A canonical two-component system consists of a homodimeric sensor histidine kinase (HK) and its cognate response regulator (RR). In the phosphotransfer reaction, the phosphate is relayed to a conserved aspartate residue within a receiver (REC) domain of the RR. By pursuing an integrated biochemical and structural strategy, we show that despite close homology, Agp1 acts as a histidine kinase whereas DrBphP functions as a light-activated phosphatase. Our results now settle this long-standing debate and show that DrBphP is a biochemically active protein that dephosphorylates the DrRR, rather than phosphorylating it.

As DrBphP and Agp1 strikingly differed in their enzymatic activity and interactions, we next asked whether these differences could be explained by the structure of the interface between the DHp and RR. To model this interface with confidence, we solved the crystal structure of the response regulator from D. radiodurans (DrRR) at 2.1 Å resolution (see Table 1 for crystallographic statistics). The protein, which consists only of a receiver (REC) domain, crystallized in the tetragonal P41212 space group with four monomers in the asymmetric unit. Overall, the structure of the DrRR is highly similar to other reported response regulators. It contains the structural features and the conserved residues critical for its receiver function in two-component signaling. Notably, the crystal structure of DrRR contained Ca2+ instead of Mg2+ ions found in other response regulator structures. The Ca2+ ions played a central role in this crystal form, as their replacement with Mg2+ did not allow crystal formation. Although Ca2+ is chemically similar to Mg2+, its larger size leads to diffuse coordination of the ion in the active sites and 45% higher B-factors compared to Mg2+ ions modeled at the same sites. In each case, the Ca2+ ions are hexagonally coordinated to surrounding atoms, which involve water molecules, the side chains of Glu15, Asp16, Asn17, the phospho-accepting Asp66, and the main-chain oxygen of Asn68. Given its presence in the DrRR crystal structure, we tested the effects of Ca2+ in the DrBphP activity and DrRR binding. We discovered that although the DrBphP/DrRR interaction was slightly stronger in the presence of Ca2+, the DrBphP enzymatic activity was lost.

>MASMTGGQQMGRGSMPERASVPLRLLLVEDNAADIFLMEMALEYSSVHTELLVARDGLEALELLEQAKTGGPFPDLILLDLNMPRVDGFELLQALRADPHLAHLPAIVLTTSNDPSDVKRAYALQANSYLTKPSTLEDFLQLIERLTAYWFGTAAIPQTYQPQLEHHHHHH[4x]>[2x]GSMANIAVQRIKREFKEVLKSEETSKNQIKVDLVDENFTELRGEIAGPPDTPYEGGRYQLEIKIPETYPFNPPKVRFITKIWHPNISSVTGAICLDILKDQWA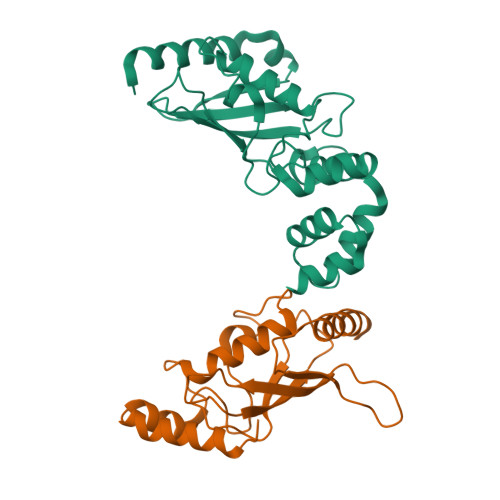AAMTLRTVLLSLQALLAAAEPDDPQDAVVANQYKQNPEMFKQTARLWAHVYAGAPVSSPEYTKKIENLCAMGFDRNAVIVALSSKSWDVETATELLLSN;>GSMSGIALSRLAQERKAWRKDHPFGFVAVPTKNPDGTMNLMNWECAIPGKKGTPWEGGLFKLRMLFKDDYPSSPPKCKFEPPLFHPNVYPSGTVCLSILEEDKDWRPAITIKQILLGIQELLNEPNIQDPAQAEAYTIYCQNRVEYEKRVRAQAKKFAPS[2x]>VRRDRAPPERGGAGTSQDGTSKNWFKITIPYGRKYDKAWLLSMIQSKSSVPFTPIEFHYENTRAQFFVEDASTASALKAVNYKILDRENRRISIIINSSAPPHTILNELKPEQVEQLKLIMSKRYDGSQQALDLKGLRSDPDLVAQNIDVVLNRRSSMAATLRIIEENIPELLSLNLSNN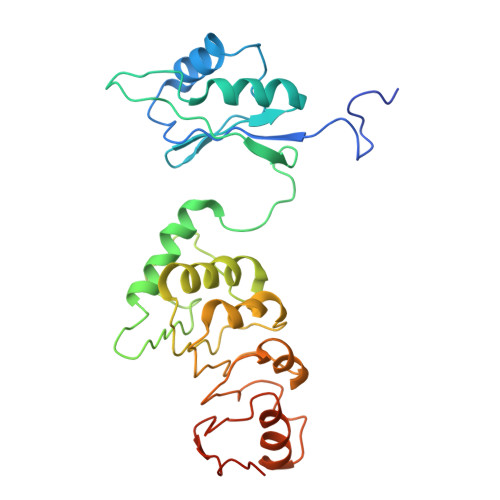RLYRLDDMSSIVQKAPNLKILNLSGNELKSERELDKIKGLKLEELWLDGNSLSDTFRDQSTYISAIRERFPKLLRLDGHELPPPIAFDVEAPTTLPP[4x]>GPLGSSKMSDVKCTSVVLLSVLQQLRVESSSKLWAQCVQLHNDILLAKDTTEAFEKMVSLLSVLLSMQGAVDINRLCEEMLDNRATLQ[4x];>GPLGSAIASEFSSLPSYAAYATAQEAY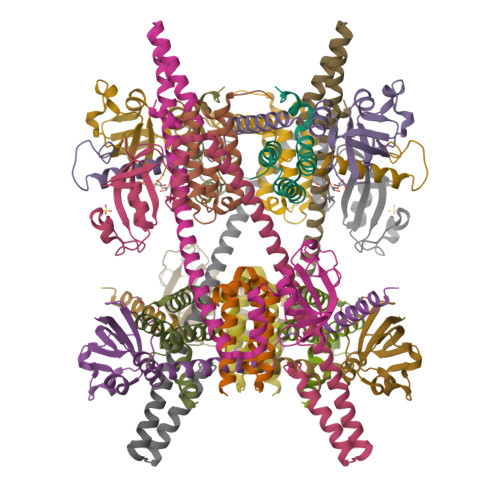EQAVANGDSEVVLKKLKKSLNVAKSEFDRDAAMQRKLEKMADQAMTQMYKQARSEDKRAKVTSAMQTMLFTMLRKLDNDALNNIINNARDGCVPLNIIPLTTAAKLMVVVPDYGTYKNTCDGNTFTYASALWEIQQVVDADSKIVQLSEINMDNSPNLAWPLIVTALRANSAVKLQ[4x]>[6x]GAMGSGASSQAACLKQILLLQLDLIEQQQQQLQAKE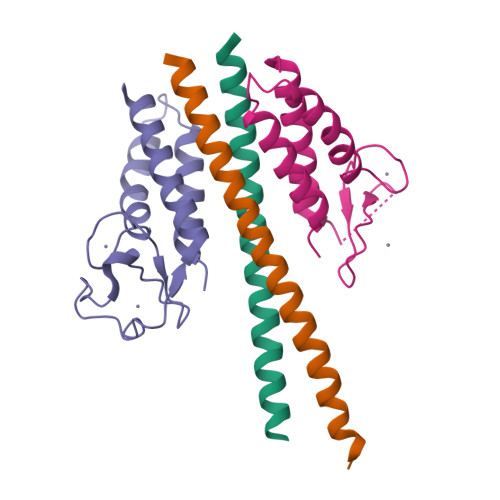KEIEELKSERDTLLARIERMERR;>MNPVNATALYISASRLVLNYDPGDPKAFTEINRLLPYFRQSLSCCVCGHLLQDPIAPTNSTCQHYVCKTCKGKKMMMKPSCSWCKDYEQFEENKQLSILVNCYKKLCEYITQTTLA[6x]>MEMTMDWKEALNWMKENLEAQDYLKAYEKPDYAVLSWWDYGNWILYVAKKAVVCNNFQAGADDAAKFFTAQSEEEAMKIVEKRKVRYVVTVEELTVKPETNKTKFIPIMQIAGYSPEYMKNKEIIDFFNKTMLYKLHVENATNLTHFRLLKN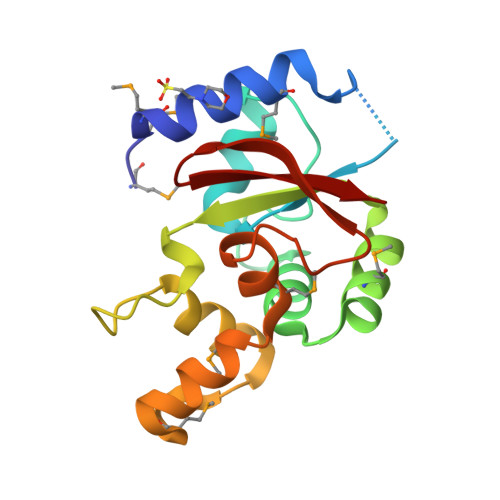FGTVKIFEVK[3x]> AADLAGKWILESSENFDDYMKAVGVGMVMRKMANAATPTQEIKIDGDSWSIKTSTTFKTTDISFTIGQEFDETTGDGRKIKTTCKIDGNAMIQDQKGSPDSILSR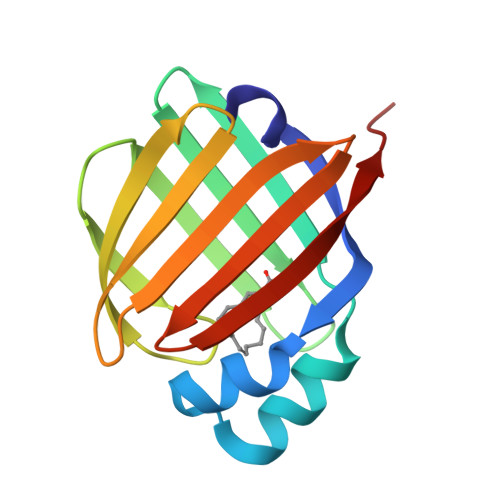EVKDGKMHMILKVNDVVCTRIYKRVDLE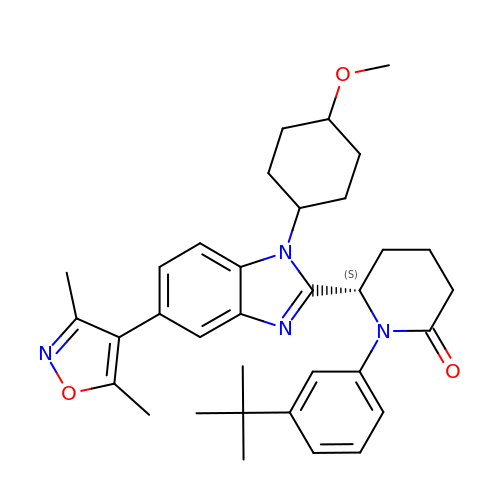(6S)-1-(3-tert-butylphenyl)-6-{(5P)-5-(3,5-dimethyl-1,2-oxazol-4-yl)-1-[(1s,4R)-4-methoxycyclohexyl]-1H-benzimidazol-2-yl}piperidin-2-one | C34 H42 N4 O3 | AITZELJGZIFAPE-NSROOHRNSA-N> MSTAITRQIVLDTETTGMNQIGAHYEGHKIIEIGAVEVVNRRLTGNNFHVYLKPDRLVDPEAFGVHGIADE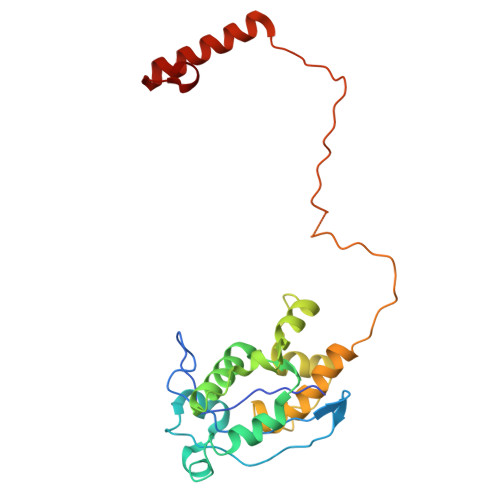FLLDKPTFAEVADEFMDYIRGAELVIHNAAFDIGFMDYEFSLLKRDIPKTNTFCKVTDSLAVARKMFPGKRNSLDALCARYEIDNSKRTLHGALLDAQILAEVYLAMTGGQLSLPLAMEGETQQQQGEATIQRIVRQASKLRVVFATDEEIAAHEARLDLVQKKGGSCLWRA> GSHHHHHHSSGLVPRGSFNELNAINENIRDDLSALLKSDFFKYFRLDLYKQCSFWDANDGLCLNRACSVDVVEDWDTLPEYWQPEILGSFNNDTMKEADDSDDECKFLDQLCQTSKKPVDIEDTINYCDVNDFNGKNAVLIDLTANPERFTG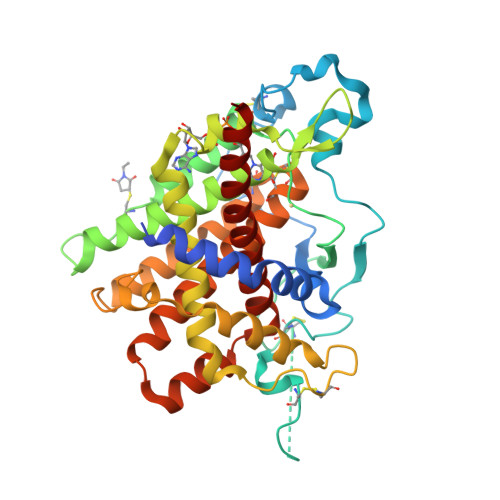YGGKQAGQIWSTIYQDNCFTIGETGESLAKDAFYRLVSGFHASIGTHLSKEYLNTKTGKWEPNLDLFMARIGNFPDRVTNMYFNYAVVAKALWKIQPYLPEFSFCDLVNKEIKNKMDNVISQLDTKIFNEDLVFANDLSLTLKDEFRSRFKNVTKIMDCVQCDRCRLWGKIQTTGYATALKILFEINDADEFTKQHIVGKLTKYELIALLQTFGRLSESIESVNMFEKMYGKRL>[2x]MASWSHPQFEKGAMQIRADFDSGNIQVIDASDPRRIRLAIRPDLASQHFQWFHFKVEGMAPATEHCFTLVNAGQSAYSHAWSGYQAVASYDGERWFRVPSQYDADGLHFQLEPEESEVRFAYFEPYSRERHARLVERALGIEGVE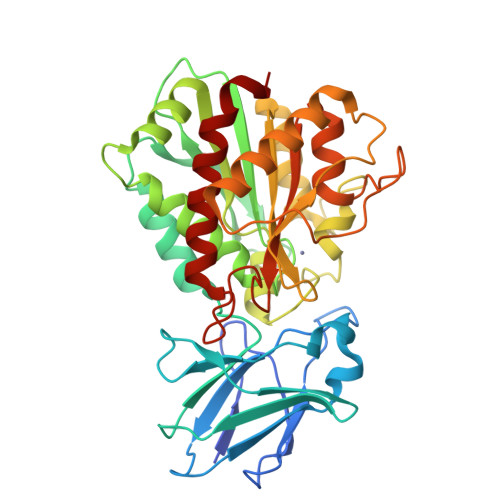RLAVGTSVQGRDIELLRVRRHPDSHLKLWVIAQQHPGEHMAEWFMEGLIERLQRPDDTEMQRLLEKADLYLVPNMNPDGAFHGNLRTNAAGQDLNRAWLEPSAERSPEVWFVQQEMKRHGVDLFLDIHGDEEIPHVFAAGCEGNPGYTPRLERLEQRFREELMARGEFQIRHGYPRSAPGQANLALACNFVGQTYDCLAFTIEMPFKDHDDNPEPGTGWSGARSKRLGQDVLSTLAVLVDELR>MALSAEGSSGGSRGGSPKAEAASVPSWPQILGRLTDNRDLARGQAAWAMDQIMTGNARPAQIAAFAVAMTMKAPTADEVGELAGVMLSHAHPLPADTVPDDAVDVVGTGGDGVNTVNLSTMAAIVVAAAGVPVVKHGNRAASSLSGGADTLEALGVRIDLGPDLVARSLAEVGIGFCFAPRFHPSYRHAAAVRREIGVPTVFNLLGPLTNPARPRAGLIGCAFADLAEVMAGVFAARRSSVLVVHGDDGLDELTTTTTSTIWRVAAGSVDKLTFDPAGFGFARAQLDQLAGGDAQANAAAVRAVLGGARGPVRDAVVLNAAGAIVAHAGLSSRAEWLPAWEEGLRRASAAIDTGA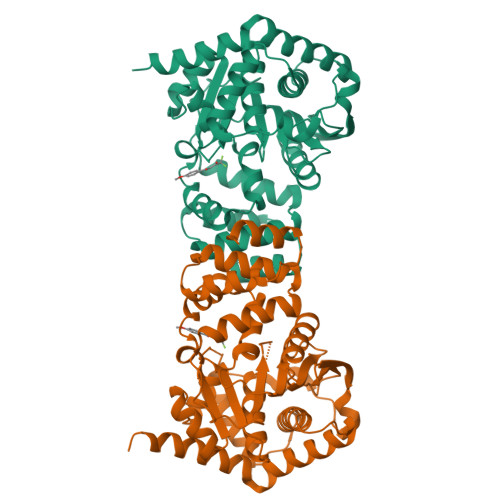AEQLLARWVRFGRQILEHHHHHH[2x]>MHHHHHHENLYFQGAVETLQGKAATGELLEKSVNTIRFLAIDAVEKANSGHPGLPMGCAPMGHVLYDEVMRYNPKNPYWFNRDRFVLSAGHGCMLQYALLHLAGYDSVKEEDLKQFRQWGSRTPGHPENFETPGVEVTTGPLGQGIANAVGLALAEKHLAARFNKPDSEIVDHYTYVILGDGCQMEGIANEACSLAGHWGLGKLIAFYDDNHISIDGDTEIAFTEDVSTRFEALGWHTIWVKNGNTGYDDIRAAIKEAKAVTDKPTLIKVTTTIGFGSPNKANSYSVHGSALGAKEVEATRQNLGWPYDTFFVPEDVKSHWSRHTPEGAALEADWNAKFAEYEKKYADDAATLKSIITGELPTGWVDALPKYTPESPGDATRNLSQQCLNALANVVPGLIGGSADLASSNMTLLKMFGDFQKDTAEERNVRFGVREHGMGAICNGIALHSPGFVPYCATFFVFTDYMRGAMRISALSEAGVIYVMTHDSIGLGEDGPTHQPIEHLVSFRAMPNILMLRPADGNETAGAYKVAVLNRKRPSILALSRQKLPHLPGTSIEGVEKGGYTISDNSTGNKPDLIVMGTGSELEIAAKAADELRKEGKTVRVVSFVSW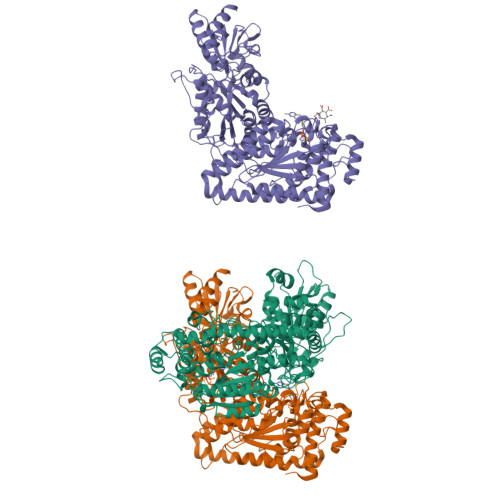ELFDEQSDEYKESVLPAAVTARISIEAGSTLGWQKYVGAQGKAIGIDKFGASAPAGTIYKEYGITVESIIAAAKSF[3x]> GPLGSMSQSNRELVVDFLSYKLSQKGYSWSQMAAVKQALREAGDEFELRYRRAFSDLTSQLHITPGTAYQSFEQVVNELFRDGVNWGRIVAFFSFGGALCVESVDKEMQVLVSRIASWMATYLNDHLEPWIQENGGWDTFVELYGN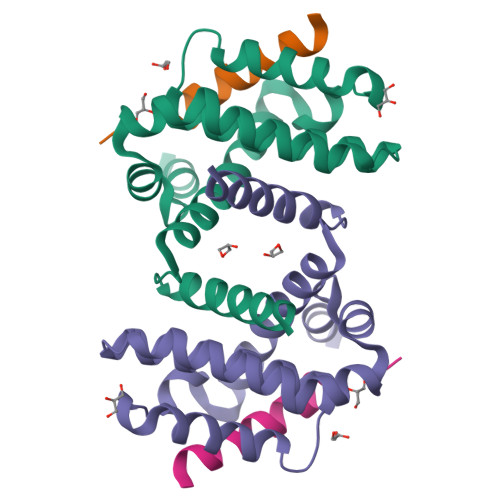NAAAESRKGQER;> LPLQPSSTMGQVGRQLAIIGDDINRRYDSEFQTM In this study, we determined the crystal structures of E. coli (S)-ureidoglycolate dehydrogenase AllD, which forms oxalurate in the presence of NAD+. This structure represents a metabolic branch point enzyme during (S)-ureidoglycolate utilization, which is the end product of purine catabolism common to plants, as well as some bacteria and fungi. (S)-Ureidoglycolate dehydrogenase AllD belongs to one of eight clades of l-sulfolactate dehydrogenase-like superfamily. The dimeric structure observed in the asymmetric unit represents the functional unit of AllD, consistent with size-exclusion chromatography, in which AllD eluted as a dimer.

In the monomer, AllD has 10 α-helices and 13 β-strands, which fold into three distinct domains. Domain I contains N- and C-terminal regions and consists of a four-helix bundle (α1, α2, α3, and α10), two antiparallel short β-strands (β1 and β13), and helix α9. Domain II is the central folding unit, with seven β-strands (β2–β3–β4–β12–β5–β8–β9 in order) and four α-helices (α4, α5, α7, and α8). Domain III is made up of loops, one helix (α6), and two short β-strands. Overall, Domains I and III, which protrude from Domain II and face each other, are localized on opposite sides of the central β-sheet in Domain II, and these domain orientations generate the inter-domain interface on the top of the central β-sheet surrounded by Domains I and III. First, conformational differences were investigated between two subunits of AllD in the apo form. This analysis resulted in a root-mean-square deviation (rmsd) of 0.45 Å for 315 corresponding Cα atoms, and these differences were evenly distributed throughout the structure, indicating that the structure of subunit A and B are essentially identical. The apo structure differed from both the binary and ternary complex by rmsd values of 0.54 Å for 337 Cα atoms. Although the rmsd values between the apo form and the two complexes were not significant, large differences are localized only in Domain III. Structural homology searches using the program DALI with subunit A of AllD in its apo form as a search model indicated nine structures in this family, with Z scores of 36–54 and rmsd values of 0.7–2.7 Å for Cα atoms.

>GHMKISRETLHQLIENKLCQAGLKREHAATVAEVLVYADARGIHSHGAVRVEYYAERISKGGTNREPEFRLEETGPCSAILHADNAAGQVAAKMGMEHAIKTAQQNGVAVVGISRMGHSGAISYFVQQAARAGFIGISMCQSDPMVVPFGGAEIYYGTNPLAFAAPGEGDEILTFDMATTVQAWGKVLDARSRNMSIPDTWAVDKNGVPTTDPFAVHALLPAAGPKGYGLMMMIDVLSGVLLGLPFGRQVSSMYDDLHAGRNLGQLHIVINPNFFSSSELFRQHLSQTMRELNAITPAPGFNQVYYPGQDQDIKQRKAAVEGIEIVDDIYQYLISDALYNTSYETKNPFAQ[2x]> MRLKVKQSSANVHSELTAAVGWNVWNELFTCSDDQTIHKWNMLGEPEQKVSTLDAYFTDMHWYPVSSKKTQAGGTDVFAVACTDGSVKILSRTGRVEKSIEGHKGACISLRWSYDGTALATAGEDGSVKIWSRNGMLRSTLAQADSPVYSIVWAYDCDQLCYCTGSNVVIKSLSSNAKQNAWKAHDGVVLKVDWSPINHLIITGGEDCKYKVWDSFGRLLFQSGLFDYPVTSVAWAPSGELFAVGGFNTLQLCDRMGWAYSKIHLNDTGSIMTLSWTADSTQLAGGGGSGGVVFGQVVDLALEDGKMQVTVVDDMRIVVNDILNENADELPEFRDRVIKVSLGYGYLIVATATQCHVYNTTNLGTPHIFDLKDTVTLLLQAERHFLLLDNSAGIQIYTYEGRQICNPRFQGLRTELLNAQMITLSNDTIAVLDQQASGTTVRFFDTAQGRPVGEPWQHTLEVKEIALSQAGTINDRQLIVIDRNRDLYLLPVMKRHVAKLAAMCDSARWHDSTAMLSAMVDQRLCVWYYPSEVYVDKDLLAKTRYTKSDSDFGKSAQIQLFAGNRCLVRRSDGVLVSAATSPYPAVLYDMIRKQQWDKATRLCRFIKDPTMWATLAAMAMAAKELNTAEVAFAAIDEVDKTHFVRKVKQIPTEEGRNAELAVYRRKPEEGESILLQAGLVFRAIKLNIKLFNWERALDLATQHKQHQDTVLWYRQQFLKNAKLAESITRFMQMNESVVVDQAAVKKKIEEERIKESQRPGAKRYVHHHHHH

With only very few exceptions, cilia are built by intraflagellar transport (IFT), the bi-directional movement of proteinaceous material sandwiched between the microtubule (MT)-based axoneme and the ciliary membrane. The IFT particle consists of a six subunit IFT-A and a 16 subunit IFT-B complex, with the latter further divided into a 10 subunit IFT-B1 and a 6-subunit IFT-B2 sub-complex. Here, we present the crystal structure of CrIFT80 to show an unusual N-terminal double β-propeller followed by α-solenoid structure. We show that the N-terminal β-propeller tethers IFT80 to the IFT complex via direct binding to the calponin-homology (CH) domain of IFT38 (also known as CLUAP1, FAP22, DYF-3, Qilin or PIFTA1) whereas the C-terminal domain is required for IFT80 dimerization.

When crystals were later obtained for fl IFT80 diffracting to 1.8 Å resolution, this partial model was used in molecular replacement to finalize the IFT80 structure. In the crystal structure, IFT80 adopts the fold of two consecutive seven bladed β-propellers followed by an alpha-solenoid extension of 4 α-helices. These helices organize into two tetratricopeptide (TPR)-like repeats, and are held in position via interactions with an extension of blade 6 of BP2. Although the fl IFT80 protein was crystallized (verified by mass spectrometry), the C-terminal 126 residues have no visible electron density and are presumably disordered in the crystal. BP1 adopts the fold of a canonical seven bladed β-propeller where the N-terminal residues contribute the first β-strand to blade 7, effectively closing the β-propeller by a zipper-like mechanism. Firstly, in the IFT80 structure, the most C-terminal β-strand of BP1 connects to BP2 as one long continuous β-strand. Inspection of the crystal packing of the IFT80 structure presented here revealed an IFT80 homo-dimer organized around a crystallographic 2-fold axis. The unusual position of the C-terminal BP2 and α-helical domains outlined above and shown in Figure 2 allows IFT80 to homo-dimerize via an extended interaction interface contributed by BP2 and the α-helical C-terminal domain. Taken together, the entire interaction interface between two IFT80 monomers (1x ‘interface 1’ and 2x ‘interface 2’) has a combined buried surface area of ~1200 Å2.>GMVFQHDIYAGQQVLVTGGSSGIGAAIAMQFAELGAEVVALGLDADGVHAPRHPRIRREELDITDSQRLQRLFEALPRLDVLVNNAGISRDREEYDLATFERVLRLNLSAAMLASQLARPLLAQRGGSILNIASMYSTFGSADRPAYSASKG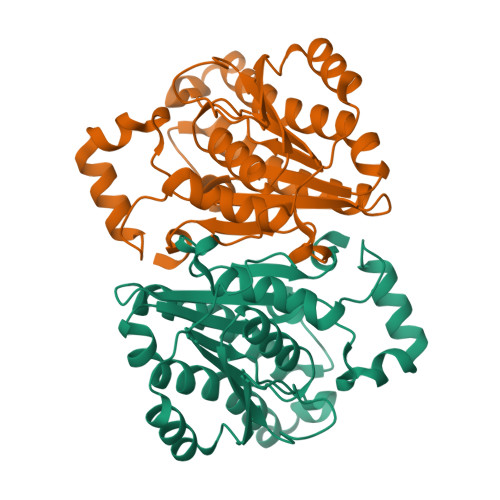AIVQLTRSLACEYAAERIRVNAIAPGWIDTPLGAGLKADVEATRRIMQRTPLARWGEAPEVASAAAFLCGPGASFVTGAVLAVDGGYLCA[2x]Csa3 family transcription factors are ancillary CRISPR-associated proteins composed of N-terminal CARF domains and C-terminal winged helix-turn-helix domains. The activity of Csa3 transcription factors is thought to be controlled by cyclic oligoadenyate (cOA) second messengers produced by type III CRISPR-Cas surveillance complexes. Here we show that Saccharolobus solfataricus Csa3a recognizes cyclic tetra-adenylate (cA4) and that Csa3a lacks self-regulating “ring nuclease” activity present in some other CARF domain proteins.

To elucidate the molecular basis for cA4 recognition by Csa3a and any conformational changes induced by cA4 binding, we co-crystallized Csa3a with cA4 and determined the structure by X-ray crystallography. Consistent with this crystal form, the asymmetric unit contains a single Csa3a homodimer, and the overall structure is largely similar to the cA4 free structure. As expected, a single cA4 molecule is bound within a two fold symmetric pocket spanning the subunit interface at the base of the Csa3a dimer. The unsaturated Gly96 main chain amines and the Arg98 side chains then mediate alternating interactions with the phosphate groups of cA4. cA4 is bound in an oval-shaped conformation with all bases present in the anti-conformation, radiating outward from the oval-shaped ribose-phosphate backbone. The β1α1 and β5β6 loops project above the floor of the cA4 binding site in an alternating pattern about the dimer axis, where they successively interdigitate between each of the four adenosine moieties. The first nucleoside is thus bound in a groove with walls formed by the β5β6 loop of subunit B and the β1α1 loop of subunit A. The conserved Gly9-Phe10 in the β1α1 loop (motif 1 of Lintner et al.) play a pivotal role. Notably, a crystal contact with a neighboring asymmetric unit results in a cation-π interaction between Arg200 and the solvent-exposed adenine ring of the fourth nucleotide. Local to the cA4 binding site, the most prominent conformational changes are modest movements of the β1α1 and β2α2 loops as they move away from the dimer axis, expanding the conserved pocket to accommodate cA4. Critically, the α3 helix runs antiparallel to the C-terminal helix of the winged helix-turn-helix DNA binding domain. This small rotation of the α3 helix is, in turn, transmitted to the C-terminal helix of the wHTH domain, acting as a pivot point for an approximate 7° rotation of the wHTH domain relative to the CARF domain.

>[2x]MKSYFVTMGFNETFLLRLLNETSAQKEDSLVIVVPSPIVSGTRAAIESLRAQISRLNYPPPRIYEIEITDFNLALSKILDIILTLPEPIISDLTMGMRMINTLILLGIIVSRKRFTVYVRDEGGGSRVISFNDNTIRALMRDYSREEMKLLNVLYETKGTGITELAKMLDKSEKTLINKIAELKKFGILTQKGKDRKVELNELGLNVIKLNK4-nitrophenyl alpha-D-6-sulfoquinovoside | 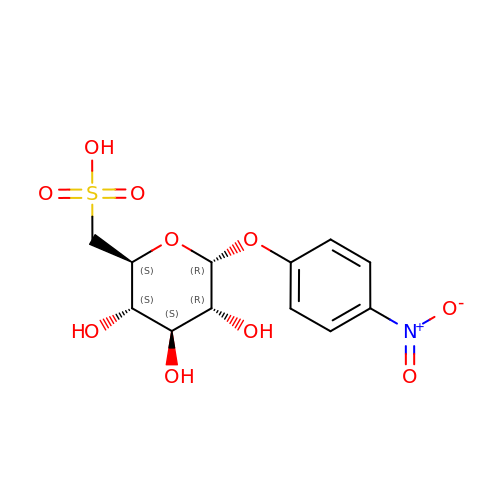C12 H15 N O10 S | JRVQBBIDMNDOQV-ZIQFBCGOSA-N3-{(4E)-4-[(1-methyl-1H-imidazol-5-yl)methylidene]-3,4-dihydro-2H-pyrrol-5-yl}pyridine | C14 H14 N4 | 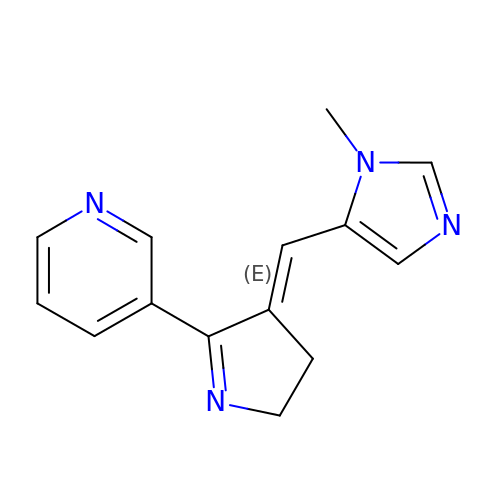JNBFHHNJEVTWBO-YRNVUSSQSA-N> SLSNKLTLDKLDVKGKRVVMRVDFNVPMKNNQITNNQRIKAAVPSIKFCLDNGAKSVVLMSHLGRPDGVPMPDKYSLEPVAVELKSLLGKDVLFLKDCVGPEVEKACANPAAGSVILLENLRFHVEEEGKGKDASGNKVKAEPAKIEAFRASLSKLGDVYVNDAFGTAHRAHSSMVGVNLPQKAGGFLMKKELNYFAKALESPERPFLAILGGAKVADKIQLINNMLDKVNEMIIGGGMAFTFLKVLNNMEIGTSLFDEEGAKIVKDLMSKAEKNGVKITLPVDFVTADKFDENAKTGQATVASGIPAGWMGLDCGPESSKKYAEAVTRAKQIVWNGPVGVFEWEAFARGTKALMDEVVKATSRGCITIIGGGDT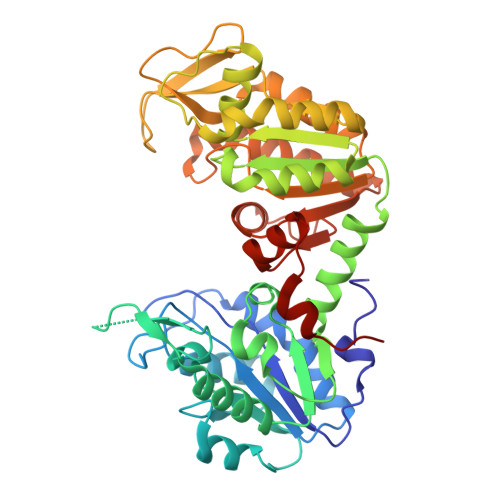ATCCAKWNTEDKVSHVSTGGGASLELLEGKVLPGVDALSNILE>GIDPFTMTSQNNQELENKLPIAKQPCPVNSYNEWDALEEVIVGSVEGAMLPALEPINKWTFPLE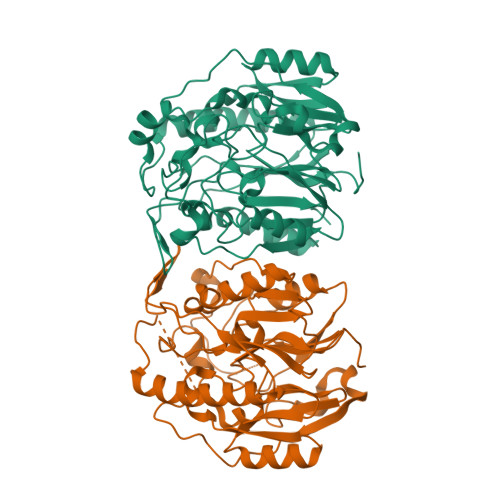ELASAQKVLFETGGIPYPPEMIAVAHKELNEFIHILEAEGVKVRRVKPVDFFASFSTPAWQVRSGFCAANPRDVFLVIGNEIIEAPMADRNRYFEAWAYRDLLKEYFQAGAKWTAAPKPQLFDAQYDFNFQFPQTGEPSRFVVTEFEPTFDAADFVRCGRDIFGQKSHVTNSLGIEWLQRHLEDEYRIHIIESQCPEALHIDTTLMPLAPGKILVNPEFVDVNKLPKILKSWDILVAPYPNHIPQNQLRLVSEWAGLNVLMLDEERVIVEKKQEPMIKALKDWGFKPIVCSFESYYPFLGSFHCATLDVRRRGTLQSYF[2x]Poliovirus (PV) is the causative agent of poliomyelitis, a highly infectious disease, which can cause paralysis and can be fatal. Mature PV virions are ~30 nm diameter icosahedral capsids comprising 60 copies of VP1-VP420. Empty capsids (ECs), which are also produced during infection, are antigenically indistinguishable from mature viral particles but do not contain viral genome and do not cleave VP022. ECs have potential as virus-like particle (VLP) vaccines to replace the current PV vaccines; however, recombinantly expressed wt ECs are inherently unstable and readily convert to an expanded form.

Detailed structural analyses and comparison of the PV2-SC6b and PV2-SC5a VLPs from bioreactor production were performed by single particle cryo-EM. Data were collected as described in “Methods”. Data processing yielded a final set of 113,853 particles for PV2-SC6b and 147,409 particles for PV2-SC5a, and icosahedral reconstructions of 2.4 Å and 2.1 Å resolution, respectively. The structures confirm that both PV2 VLPs adopt a homogeneous D Ag conformation, with negligible or no particles observed in C Ag form. The quality of the cryo-EM electron potential maps is sufficient to resolve the stabilising mutations and confirm that they introduce no significant perturbations to the structure and do not impinge on the antigenic surface of the particle. Based on the extent of the observed electron potential map in the VP1 pockets of both PV2-SC6b and PV2-SC5a, a sphingosine lipid moiety of carbon length 18 was modelled into the maps. For PV2-SC6b the mutation in subunit VP4 I57V (I57V in VP0) and for PV2-SC5a the mutation in subunit VP1 T41I, were in disordered regions of the map and were not modelled. Unexpectedly, in the PV2-SC6b structure reported here from bioreactor production an apparent disulphide bond is observed between residues Cys130 and Cys326 of the VP0 subunit (equivalent to Cys61 and Cys257, respectively, of the mature VP2 peptide). Whilst these cysteine residues are conserved across all types of PV, the bond between them has not been seen in any previously reported poliovirus structure and is not formed in either the bioreactor produced PV2-SC5a reported in this study, or in previously determined structures of PV2-SC6b from mammalian and insect cell expression. The yield of PV1-SC6b D Ag was increased by ~3-fold and that of PV3-SC8 was improved ~2-fold, whereas the yield of PV2-SC6b was ~10-fold greater in comparison to flask-based expression.

> GLGDLIEGVVEGVTRNALTPLTPANNLPDTQSSGPAHSKETPALTAVETGATNPLVPSDTVQTRHVIQKRTRSESTVESFFARGACVAIIEVDNDAPTKRASKLFSIWKITYKDTVQLRRKLEFFTYSRFDMELTFVVTSNYTDANNGHALNQVYQIMYIPPGAPIPGKWNDYTWQTSSNPSLFYTYGAPPARISVPYVGIANAYSHFYDGFAKVPLAGQASTEGDSLYGAASLNDFGSLAVRVVNDHNPTKLTSKIRVYMKPKHVRVWCPRPPRAVPYYGPGVDYKDGLAPLPEKGLTTY;> MGAQVSSQKVGAHENSNRAYGGSTINYTTINYYRDSASNAASKQDFAQDPSKFTEPVKDVLIKTAPTLNSPNIEACGYSDRVMQLTLGNSTITTQEAANSVVAYGRWPEYIKDSEANPVDQPTEPAVAACRFYTLDTVTWRKESRGWWWKLPDALKDMGLFGQNMFYHYLGRAGYTVHVQCNASKFHQGALGVFAVPEMCLAGDSTTHMFTKYENANPGEKGGEFKGSFTLDTNATNPARNFCPVDYLFGSGVLAGNAFVYPHQIINLRTNNCATLVLPYVNSLSIDSMTKHNNWGIAILPLAPLDFATESSTEIPITLTIAPMCCEFNGLRNITVPRTQ;> GLPVLNTPGSNQYLTADNYQSPCAIPEFDVTPPIDIPGEVRNMMELAEIDTMIPLNLTNQRKNTMDMYRVELNDAAHSDTPILCLSLSPASDPRLAHTMLGEILNYYTHWAGSLKFTFLFCGSMMATGKLLVSYAPPGAEAPKSRKEAMLGTHVIWDIGLQSSCTMVVPWISNTTYRLTINDSFTEGGYISMFYQTRVVVPLSTPRKMDILGFVSACNDFSVRLLRDTTHISQEAMPQ Bacterial AAA+ proteases are composed of a AAA+ partner (e.g., ClpC) and an associated peptidase (e.g., ClpP). They represent ATP-fuelled and self-compartmentalized proteolytic machines that are crucial for stress resistance and virulence. ClpC requires cooperation with adaptor proteins such as MecA for activation and complex formation with ClpP. Here, we present the cryo-EM structure of the MecA/ClpC/ClpP complex from the major pathogen Staphylococcus aureus.

To determine the cryo-EM structure of the central ClpP/ClpC/MecA protease from Staphylococcus aureus, we assembled the components in vitro in the presence of 2 mM ATPγS and assessed complex formation by negative stain. The MecA/ClpC/ClpP complex is composed of several layers: (i) a mobile regulatory subcomplex encompassing MecA and interacting with the N-terminal (NTD) and middle (MD) domains of ClpC, (ii) the two ATPase rings of ClpC formed by AAA-1 and AAA-2 domains and (iii) a well-defined double-heptameric ClpP barrel. The overall map of MecA/ClpC/ClpP was refined in CryoSPARCv4.5 to an average resolution of 2.9 Å, but it is resolved at very different levels of detail as shown by the local resolution that ranges from 2 Å in the ClpP part to 9 Å in the MecA-ClpC interaction region. ClpC forms a shallow right-handed spiral with protomer a located at the lowest position of the staircase. Two substrate peptides are visible, trapped inside the ClpC channel, each of 8 aa, one grabbed by the AAA-1 pore loops of protomers a, b, c and d, one by the AAA-2 pore loop of protomers b, c, d and e. The interface between ClpP and ClpC is mediated by two main interaction points: the ClpC P-loops and the ClpP N-terminal β-hairpins. The ClpP NTD β-hairpins contact the ClpC inner channel more on one side of the ring involving ClpC subunits a-e and ClpP protomers Pa-Pf. In summary, the AAA-2 ring can be separated into an inactive half, including subunits f-b and an active half represented by ATPase-poised subunits c-e. In the ClpC AAA-1 ring, the nucleotide states are similar to AAA-2, yet they are shifted relative to AAA-2 by one subunit (a: ADP, b-e ATP bound, f: empty). ClpP β-hairpins establish a tight contact with the subunits at the interface between the active and the inactive half of the AAA-2 ring.

>[6x]MRIERVDDTTVKLFITYSDIEARGFSREDLWTNRKRGEEFFWSMMDEINEEEDFVVEGPLWIQVHAFEKGVEVTISKSKNEDMMNMSDDDATDQFDEQVQELLAQTLEGEDQLEELFEQRTKEKEAQGSKRQKSSARKNTRTIIVKFNDLEDVINYAYHSNPITTEFEDLLYMVDGTYYYAVYFDSHVDQEVINDSYSQLLEFAYPTDRTEVYLNDYAKIIMSHNVTAQVRRYFPETTE;>MNLIPTVIETTNRGERAYDIYSRLLKDRIIMLGSQIDDNVANSIVSQLLFLQAQDSEKDIYLYINSPGGSVTAGFAIYDTIQHIKPDVQTICIGMAASMGSFLLAAGAKGKRFALPNAEVMIHQPLGGAQGQATEIEIAANHILKTREKLNRILSERTGQSIEKIQKDTDRDNFLTAEEAKEYGLIDEVMVPETK[14x];>[6x]MLFGRLTERAQRVLAHAQEEAIRLNHSNIGTEHLLLGLMKEPEGIAAKVLESFNITEDKVIEEVEKLIGHGQDHVGTLHYTPRAKKVIELSMDEARKLHHNFVGTEHILLGLIRENEGVAARVFANLDLNITKARAQVVKALGNPEMSNKNAQASKSNNTPTLDSLARDLTVIAKDGTLDPVIGRDKEITRVIEVLSRRTKNNPVLIGEPGVGKTAIAEGLAQAIVNNEVPETLKDKRVMSLDMGTVVAGTKYRGEFEERLKKVMEEIQQAGNVILFIDELHTLVGAGGAEGAIDASNILKPALARGELQCIGATTLDEYRKNIEKDAALERRFQPVQVDEPSVVDTVAILKGLRDRYEAHHRINISDEAIEAAVKLSNRYVSDRFLPDKAIDLIDEASSKVRLKSHTTPNNLKEIEQEIEKVKNEKDAAVHAQEFENAANLRDKQTKLEKQYEEAKNEWKNAQNGMSTSLSEEDIAEVIAGWTGIPLTKINETESEKLLSLEDTLHERVIGQKDAVNSISKAVRRARAGLKDPKRPIGSFIFLGPTGVGKTELARALAESMFGDDDAMIRVDMSEFMEKHAVSRLVGAPPGYVGHDDGGQLTEKVRRKPYSVILFDEIEKAHPDVFNILLQVLDDGHLTDTKGRTVDFRNTIIIMTSNVGAQELQDQRFAGFGGSSDGQDYETIRKTMLKELKNSFRPEFLNRVDDIIVFHKLTKEELKEIVTMMVNKLTNRLSEQNINIIVTDKAKDKIAEEGYDPEYGARPLIRAIQKTIEDNLSELILDGNQIEGKKVTVDHDGKEFKYDIAEQTSETKTPSQA>CGTSNGGQNTSPSTSSSSAKGEASALPKGQTITVWSWQTGPELQDVKQIAAQWAKAHGDKVIVVDQSSNPKGFQFYATAARTGKGPDVVFGMPHDNNGVFAEEGLMAPVPSGVLNTGLYAPNTIDAIKVNGTMYSVPVSVQVAAIYYNKKLVPQPPQTWAEFVKDANAHGFMYDQANLYFDYAIIGGYGGYVFKDNNGTLDPNNIGLDTPGAVQAYTLMRDMVSKYHWMTPSTNGSIAKAEFLAGKIGMYVSGPWDTADIEKAKIDFGVTPWPTLPNGKHAT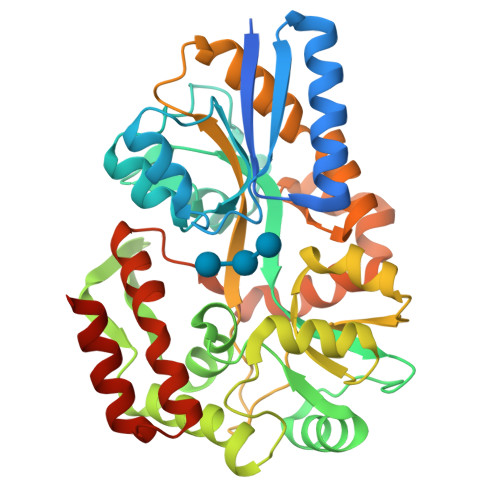PFLGVITAFVNKESKTQAADWSLVQALTSAQAQQMYFRDSQQIPALLSVQRSSAVQSSPTFKAFVEQLRYAVPMPNIPQMQAVWQAMSILQNIIAGKVSPEQGAKDFVQNIQKGIMAQGS[2x]>MGSSHHHHHHSQDPNSKIIIDTDPGIDDSVAILMAFQMPGVQVLGLTTIFGNCTTEHATRNALILCEKASHLEVPVAEGSHEPLKGGKPHVADFVHGPDGLGNVDLPDPTIKKVEESATDFLVDKVSRFPGEVSVLALGPLTNIALAIKKDPSFVKNVKKIVVLGGAFFAAGNATPSAEANIH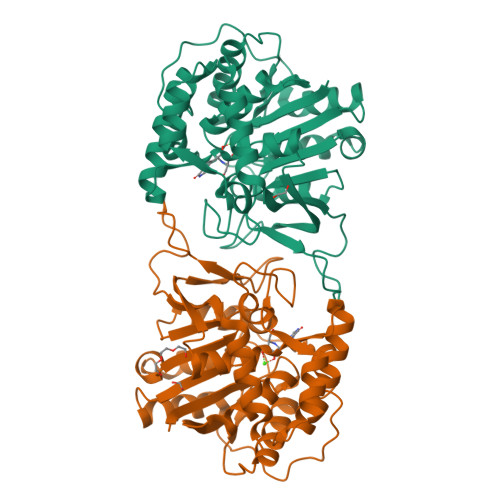SDPEAADMVFTSGADIYVVGLNITTQVSFTDKDLLELRNSQGKYAQFLCDVCKFYLDWHTESYGAPVIFLHDPVSFAALVRPELFTFKKGVVRVETQGICVGHTSMDMLLKKWNSENPWTGYSPISVAWTVDVPKVVAFVKELVTKP[2x]>GEDSLTKQPEEVFDVLEKLGEGSYGSVFKAIHKESGQVVAIKQVPVESDLQEIIKEISIMQQCDSPYVVKYYGSYFKNTDLWIVMEYCGAGSVSDIIRLRNKTLIEDEIATILKSTLKGLEYLHFMRKIHRDIKAGNILLNTEGHAKLADFGVAGQLTDTMAKRNTVIGTPFWMAPEVIQEIGYNCVADIWSLGITSIEMAEGKPPYADIHPMRAIFMIPTNPPPTFRKPELWSDDFTDFVKKCLVKNPEQRATATQLLQHPFIKNAKPVSILRDLITEA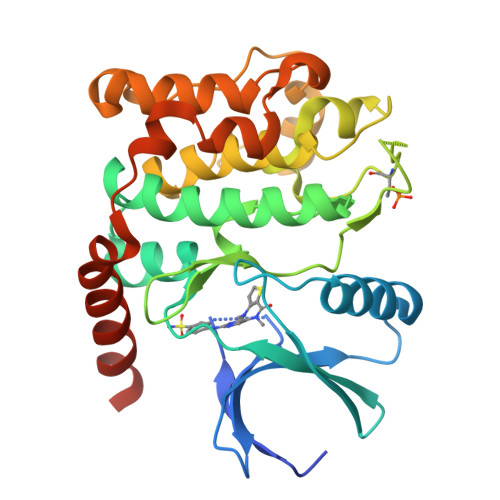MEIKAKRHEEQQRELEEE[2x]> MILSDKDIIDYVTSKRIIIKPFNKDFVGPCSYDVTLGDEFIIYDDEVYDLSKELNYKRIKIKNSILVCPLNYNLTEEKINYFKEKYNVDYVVEGGVLGTTNEYIELPNDISAQYQGRSSLGRVFLTSHQTAGWIDAGFKGKITLAIVAFDKPVILYKNQRIGQLIFS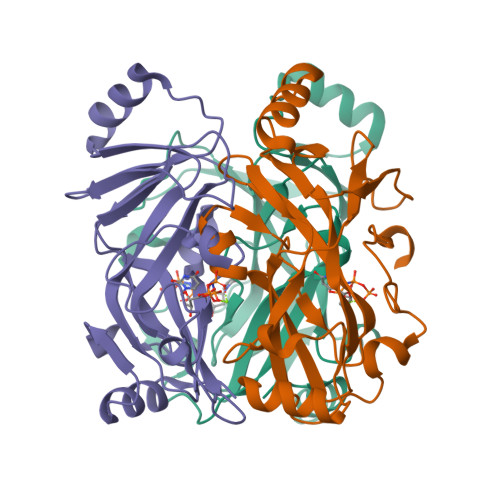KLLSPADVGYSERKTSKYAYQKSVMPSLIHLDNHKKD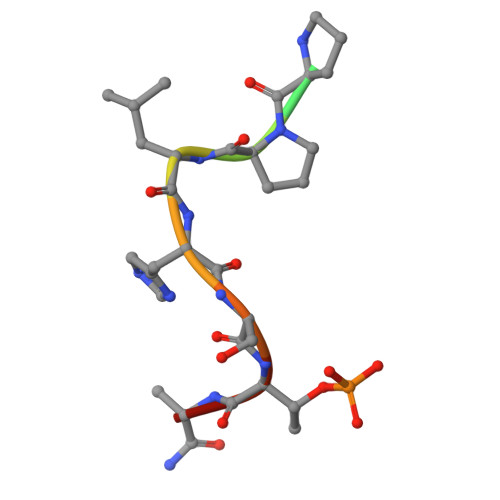> XLDPPLHSTAX> TENIISVDHLTYQYDENQA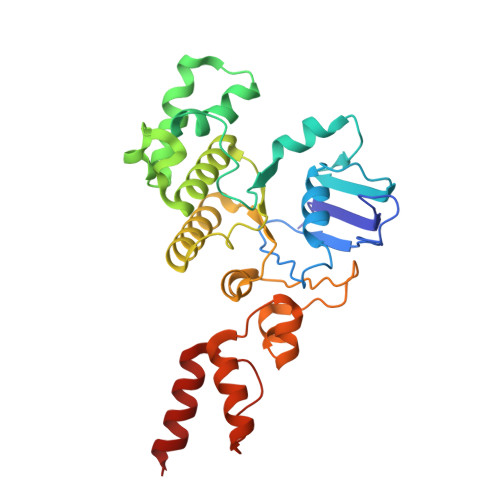PALTDVSFTVHAGEWLAIVGHNGSGKSTLAKSLDGLLPFTQGSVTVGGITLTPETVWQVREQIGMIFQNPDNQFVGATVEDDVAFGLENRQISRDEMVPRVQAALAQVGMTSFAQREPSSLSGGQKQRVALAGIVAIAPKILILDEATSMLDPQGRIEMLAIVRQLRQQQNLTVISITHDIDEAASADRVLVIDDGRLVDEAVPSQIFERGTQLVEMGLDLPFTEKLKAALRQRGITPPTTYQTAAEMEEWLWQSLSNT> MAYPESLKAHLQ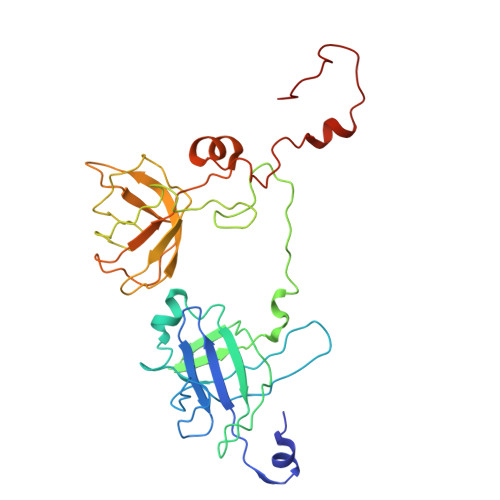GGVTTLARAWALARADGRVLGFTDHDVVLRFDGISFEPGSGMTAKAVLQGTGLSVDNTESYGALSSEAITEADLLAGRYDGAAVTVWLVNWADPAMRAVIFRGHLGEVSRGAGAFTAELRGLTAALGQEQGRIYHPRCAAVLGDGRCRFDLTKDGYALEAALGGVDEAVVLRLAEGAGFEDRWFEKGRLVVLDGAAAGLIGVVKNDRLQADGSRLIELWQRLGANPVAGDRVRIEPGCDKRAGTCRLKFDNFLNFRGFPHIPGEDWMVSYPVQSGTNDGGSLFR> VSYANAVSRAAPAVANLYTTKMVSKPSHPLFDDPMFRRFFGDNLPQQKRMESSLGSAVIMSAEGYLLTNNHVTAGADQIIVALRDGRETIAQLVGSDPETDLAVLKIDLKNLPAMTLGRSDGIRTGDVCLAIGNPFGVGQTVTMGIISATGRNQLGLNTYEDFIQTDAAINPGNAGGALVDAAGNLIGINTAIFSKSGGS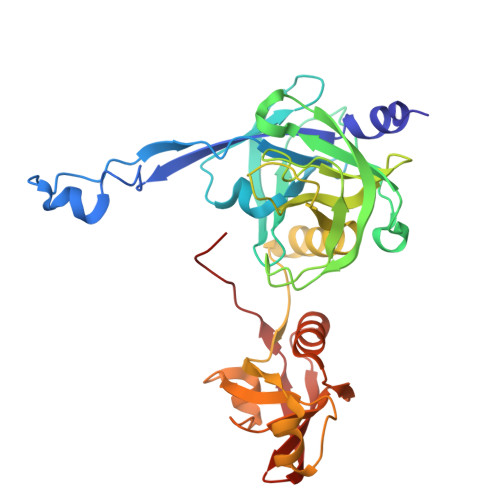QGIGFAIPTKLALEVMQSIIEHGQVIRGWLGVEVKALTPELAESLGLGETAGIVVAGVYRDGPAARGGLLPGDVILTIDKQEASDGRRSMNQVARTRPGQKISIVVLRNGQKVNLTAEVGLRPPPAPAP Vps4, a member of the type-I or meiotic clade of AAA family of proteins (ATPase associated with various activities)11 disassembles ESCRT-III polymers from membranes, which might be coupled to the membrane fission reaction itself. Proteins homologous to Vps4 and ESCRT-III are also present in the Crenarchaeota phylum of archaea where they catalyse final steps in cell division, virus budding and vesicle release. Vps4 contains an amino-terminal microtubule interacting and trafficking (MIT) domain that interacts with carboxy-terminal peptide motifs termed MIT domain-interacting motif in activated eukaryotic and archaeal ESCRT-III proteins. Here we characterized the oligomeric state of the Vps4 homologue from M. sedula (MsVps4) that belongs to the phylum Crenarchaeota.

To probe the conformation on nucleotide binding, hexameric MsVps4ΔMIT and a shorter MsVps4 construct lacking the linker region (MsVps4ΔL-MIT, residues 88–369) were crystallized in the presence of ADP and Mg2+. Both constructs crystallized with P65 helical symmetry with similar H interfaces as observed in the hexamer structure and a V interface close the to A–B interface. ADP is coordinated between the large and small ATPase domains and P-loop residues Gly141, Cys142, Gly143, Lys144 and Thr145 (located on the large ATPase domain) bind the α- and β-phosphate groups of ADP, whereas Tyr282, Arg310 and Val103 (located on the small ATPase domain) make hydrogen bonds with the sugar and the base. The base is stacked between the small and large ATPase domain in a pocket composed of residues Met146, Leu278 and Ala306. Comparison of the nucleotide-free apo structure present in the ring structure showed that ADP binding induced a 23° rotation of the small ATPase domain compared with the large one. ADP bound to MsVps4 occupies a similar position as ATPγS bound to yeast Vps4p, whereas ADP bound to yeast Vps4p penetrates less into the binding pocket. ADP binding to MsVps4 induces rotation of the small ATPase domain with respect to the large domain as reported for other Vps4 structures and ClpX4041. Our crystal structures reveal that the β′-strand at the N terminus is ordered in the ADP-bound conformation and disordered in the nucleotide-free conformation, suggesting that this conformational flexibility might be important for MIT domain orientation.

>[3x]GVPEGGEETEKAEEDIVMKEKPKVTLNEIVGLEDVKEALKEAVVYPSKRPDLFPLGWPRGILLYGPPGCGKTMIAAAVANELDSEFIHVDAASIMSKWLGEAEKNVAKIFKTARELSKKENKPAIIFIDELDALLASYTSEVGGEARVRNQFLKEMDGLADKNEISKVYVIGATNKPWRLDEPFLRRFQKRIYITLPDKAHRLELLKHYSSKVKLDPNVNLEELAELTDGYTASDIRDIVQSAHMRVVKEMFEKNLQEPRAINMDDFREVLKVRKPSVNQDMLKAYAAWHEKFKAL>XXXXXXXXXXXXXXXXXXXXXXXXXXXXXXXXXXXXXXXXXXXXXXXXXXXXXEMSQEESTRFYDQLNHHIFELVSSSDANERKGGILAIASLIGVEGGNATRIGRFANYLRNLLPSNDPVVMEMASKAIGRLAMAGDTFTAEYVEFEVKRALEWLGADRNEGRRHAAVLVLRELAISVPTFFFQQVQPFFDNIFVAVWDPKQAIREGAVAALRACLILTTQREPKEMQKPQWYRHTFEEAEKGFDETLAKEKGMNRDDRIHGALLILNELVRISSMEGERLREEMEEITQQQLVHDKYCKDLMGFGTKPRHITPFTSFQAVQPQQSNALVGLLGYSSHQGLMGFGTSPSPAKSTXXXXXXXXXXXXXXXXXXXXXXXXXRNSKNSLIQMTILNLLPRLAAFRPSAFTDTQYLQDTMNHVLSCVKKEKERTAAFQALGLLSVAVRSEFKVYLPRVLDIIRAALPPKDFAHKRQKAMQVDATVFTCISMLARAMGPGIQQDIKELLEPMLAVGLSPALTAVLYDLSRQIPQLKKDIQDGLLKMLSLVLMHKPLRHPGMPKGLAHQLASPGLTTLPEASDVGSITLALRTLGSFEFEGHSLTQFVRHCADHFLNSEHKEIRMEAARTCSRLLTPSIHLISGHAHVVSQTAVQVVADVLSKLLVVGITDPDPDIRYCVLASLDERFDAHLAQAENLQALFVALNDQVFEIRELAICTVGRLSSMNPAFVMPFLRKMLIQILTELEHSGIGRIKEQSARMLGHLVSNAPRLIRPYMEPILKALILKLKDPDPDPNPGVINNVLATIGELAQVSGLEMRKWVDELFIIIMDMLQDSSLLAKRQVALWTLGQLVASTGYVVEPYRKYPTLLEVLLNFLKTEQNQGTRREAIRVLGLLGALDPYKHKVNIGMIDQSRDASAVSLSESKSSQDSSDYSTSEMLVNMGNLPLDEFYPAVSMVALMRIFRDQSLSHHHTMVVQAITFIFKSLGLKCVQFLPQVMPTFLNVIRVCDGAIREFLFQQLGMLVSFVKSHIRPYMDEIVTLMREFWVMNTSIQSTIILLIEQIVVALGGEFKLYLPQLIPHMLRVFMHDNSPGRIVSIKLLAAIQLFGANLDDYLHLLLPPIVKLFDAPEAPLPSRKAALETVDRLTESLDFTDYASRIIHPIVRTLDQSPELRSTAMDTLSSLVFQLGKKYQIFIPMVNKVLVRHRINHQRYDVLICRIVKGYTLADEEEDPLIYQHRMLRSGQGDALASGPVETGPMKKLHVSTINLQKAWGAARRVSKDDWLEWLRRLSLELLKDSSSPSLRSCWALAQAYNPMARDLFNAAFVSCWSELNEDQQDELIRSIELALTSQDIAEVTQTLLNLAEFMEHSDKGPLPLRDDNGIVLLGERAAKCRAYAKALHYKELEFQKGPTPAILESLISINNKLQQPEAAAGVLEYAMKHFGELEIQATWYEKLHEWEDALVAYDKKMDTNKDDPELMLGRMRCLEALGEWGQLHQQCCEKWTLVNDETQAKMARMAAAAAWGLGQWDSMEEYTCMIPRDTHDGAFYRAVLALHQDLFSLAQQCIDKARDLLDAELTAMAGESYSRAYGAMVSCHMLSELEEVIQYKLVPERREIIRQIWWERLQGCQRIVEDWQKILMVRSLVVSPHEDMRTWLKYASLCGKSGRLALAHKTLVLLLGVDPSRQLDHPLPTVHPQVTYAYMKNMWKSARKIDAFQHMQHFVQTMQQQAQHAIATEDQQHKQELHKLMARCFLKLGEWQLNLQGINESTIPKVLQYYSAATEHDRSWYKAWHAWAVMNFEAVLHYKHQNQARDEKKKLRHASGANITNATTAATTAATATTTASTEGSNSESEAESTENSPTPSPLQKKVTEDLSKTLLMYTVPAVQGFFRSISLSRGNNLQDTLRVLTLWFDYGHWPDVNEALVEGVKAIQIDTWLQVIPQLIARIDTPRPLVGRLIHQLLTDIGRYHPQALIYPLTVASKSTTTARHNAANKILKNMCEHSNTLVQQAMMVSEELIRVAILWHEMWHEGLEEASRLYFGERNVKGMFEVLEPLHAMMERGPQTLKETSFNQAYGRDLMEAQEWCRKYMKSGNVKDLTQAWDLYYHVFRRISKQLPQLTSLELQYVSPKLLMCRDLELAVPGTYDPNQPIIRIQSIAPSLQVITSKQRPRKLTLMGSNGHEFVFLLKGHEDLRQDERVMQLFGLVNTLLANDPTSLRKNLSIQRYAVIPLSTNSGLIGWVPHCDTLHALIRDYREKKKILLNIEHRIMLRMAPDYDHLTLMQKVEVFEHAVNNTAGDDLAKLLWLKSPSSEVWFDRRTNYTRSLAVMSMVGYILGLGDRHPSNLMLDRLSGKILHIDFGDCFEVAMTREKFPEKIPFRLTRMLTNAMEVTGLDGNYRITCHTVMEVLREHKDSVMAVLEAFVYDPLLNWRLMDTNTKGNKRSRTRTDSYSAGQSVEILDGVELGEPAHKKTGTTVPESIHSFIGDGLVKPEALNKKAIQIINRVRDKLTGRDFSHDDTLDVPTQVELLIKQATSHENLCQCYIGWCPFW[2x];>MPNTAMKKKVLLMGKSGSGKTSMRSIIFANYIARDTRRLGATIDVEHSHVRFLGNLVLNLWDCGGLDTFMENYFTSQRDNIFRNVEVLIYVFDVESRELEKDMHYYQSCLEAILQNSPDAKIFCLVHKMDLVQEDQRDLIFKEREEDLRRLSRPLECACFRTSIWDETLYKAWSSIVYQLIPNVQQLEMNLRNFAQIIEADEVLLFERATFLVISHYQCKEQRDVHRFEKISNIIKQFKLSCSKLAASFQSMEVRNSNFAAFIDIFTSNTYVMVVMSDPSIPSAATLINIRNARKHFEKLERVDGPKHSLLMR[2x];>[2x]MSLQYGAEETPLAGSYGAADSFPKDFGYGVEEEEEEAAAAGGGVGAGAGGGCGPGGADSSKPRILLMGLRRSGKSSIQKVVFHKMSPNENLFLESTNKIYKDDISNSSFVNFQIWDFPGQMDFFDPTFDYEMIFRGTGALIYVIDAQDDYMEALTRLHITVSKAYKVNPDMNFEVFIHKVDGLSDDHKIETQRDIHQRANDDLADAGLEKLHLSFYLTSIYDHSIFEAFSKVVQKLIPQLPTLENLLNIFISNSGIEKAFLFDVVSKIYIATDSSPVDMQSYELCCDMIDVVIDVSCIYGLKEDGSGSAYDKESMAIIKLNNTTVLYLKEVTKFLALVCILREESFERKGLIDYNFHCFRKAIHEVFEVGVTSHRSCGHQTSASSLKALTHNGTPRNAI;>MNTSPGTVGSDPVILATAGYDHTVRFWQAHSGICTRTVQHQDSQVNALEVTPDRSMIAAAGYQHIRMYDLNSNNPNPIISYDGVNKNIASVGFHEDGRWMYTGGEDCTARIWDLRSRNLQCQRIFQVNAPINCVCLHPNQAELIVGDQSGAIHIWDLKTDHNEQLIPEPEVSITSAHIDPDASYMAAVNSTGNCYVWNLTGGIGDEVTQLIPKTKIPAHTRYALQCRFSPDSTLLATCSADQTCKIWRTSNFSLMTELSIKSGNPGESSRGWMWGCAFSGDSQYIVTASSDNLARLWCVETGEIKREYGGHQKAVVCLAFNDSVLG[2x];>[2x]MESEMLQSPLLGLGEEDEADLTDWNLPLAFMKKRHCEKIEGSKSLAQSWRMKDRMKTVSVALVLCLNVGVDPPDVVKTTPCARLECWIDPLSMGPQKALETIGANLQKQYENWQPRARYKQSLDPTVDEVKKLCTSLRRNAKEERVLFHYNGHGVPRPTVNGEVWVFNKNYTQYIPLSIYDLQTWMGSPSIFVYDCSNAGLIVKSFKQFALQREQELEVAAINPNHPLAQMPLPPSMKNCIQLAACEATELLPMIPDLPADLFTSCLTTPIKIALRWFCMQKCVSLVPGVTLDLIEKIPGRLNDRRTPLGELNWIFTAITDTIAWNVLPRDLFQKLFRQDLLVASLFRNFLLAERIMRSYNCTPVSSPRLPPTYMHAMWQAWDLAVDICLSQLPTIIEEGTAFRHSPFFAEQLTAFQVWLTMGVENRNPPEQLPIVLQVLLSQVHRLRALDLLGRFLDLGPWAVSLALSVGIFPYVLKLLQSSARELRPLLVFIWAKILAVDSSCQADLVKDNGHKYFLSVLADPYMPAEHRTMTAFILAVIVNSYHTGQEACLQGNLIAICLEQLNDPHPLLRQWVAICLGRIWQNFDSARWCGVRDSAHEKLYSLLSDPIPEVRCAAVFALGTFVGNSAERTDHSTTIDHNVAMMLAQLVSDGSPMVRKELVVALSHLVVQYESNFCTVALQFIEEEKNYALPSPATTEGGSLTPVRDSPCTPRLRSVSSYGNIRAVATARSLNKSLQNLSLTEESGGAVAFSPGNLSTSSSASSTLGSPENEEHILSFETIDKMRRASSYSSLNSLIGVSFNSVYTQIWRVLLHLAADPYPEVSDVAMKVLNSIAYKATVNARPQRVLDTSSLTQSAPASPTNKGVHIHQAGGSPPASSTSSSSLTNDVAKQPVSRDLPSGRPGTTGPAGAQYTPHSHQFPRTRKMFDKGPEQTADDADDAAGHKSFISATVQTGFCDWSARYFAQPVMKIPEEHDLESQIRKEREWRFLRNSRVRRQAQQVIQKGITRLDDQIFLNRNPGVPSVVKFHPFTPCIAVADKDSICFWDWEKGEKLDYFHNGNPRYTRVTAMEYLNGQDCSLLLTATDDGAIRVWKNF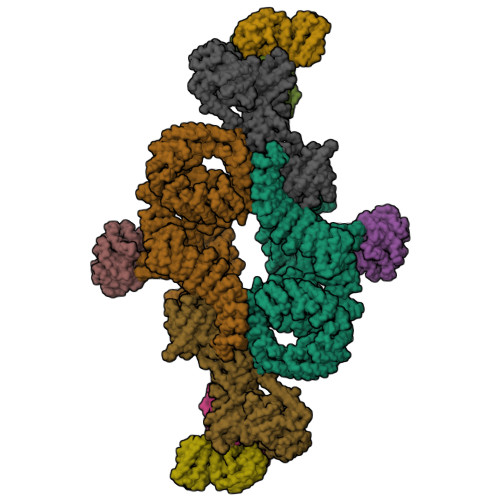ADLEKNPEMVTAWQGLSDMLPTTRGAGMVVDWEQETGLLMSSGDVRIVRIWDTDREMKVQDIPTGADSCVTSLSCDSHRSLIVAGLGDGSIRVYDRRMALSECRVMTYREHTAWVVKASLQKRPDGHIVSVSVNGDVRIFDPRMPESVNVLQIVKGLTALDIHPQADLIACGSVNQFTAIYNSSGELINNIKYYDGFMGQRVGAISCLAFHPHWPHLAVGSNDYYISVYSVEKRVR> MDQEGQPLLSKDFQQVLLATASGNNSSWTERAVLNNESTDAVKHEPALGQNDVFDLDPLSFDKWVPFLRRALDKNQLDPVIDELENSIEDNFQGLELQLLQDSQMNDKLETSIDEIANIQGMVQDTLSSEISKFQIRLSESANELIVKKQMYVNNKKISLKISEATILITKVVRILELSSKCQELITERKFFKVLQNLDSLEKLYLQEFKNYNFQFLIEIYNSIPFLQKVTKDECINLIRNSLNLNLGKNLIKVGQEFVAIYENELLPQWLETRSKMKLTNFKFNSPIEISMRDESFLAKLNLGEFFQLDDFHDSIMIFQNLNELSVLSGEFNKEYELRKTKLMYPLIWKKNKTAAYQMDSLLRGTGTTPGSTAHDVSTDDPFTQSLSLHFLQDYFLKILGFLLYDINLNKATEFILVDNNYNSTNEFWDGLMDRLSPYLSYFIDEKLKTEEDMIKLKDFLCIYVAILENFKL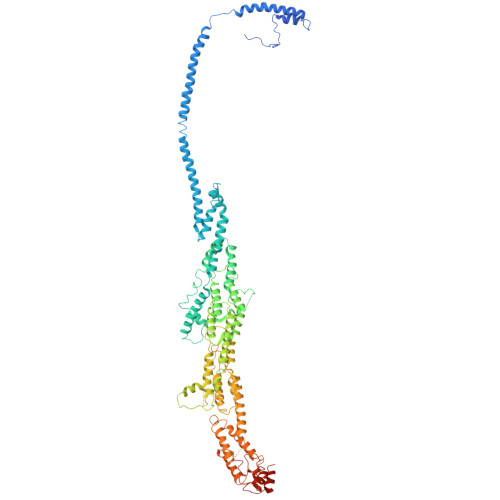NIEPLYKILVSIFEKFCSVSLRAFDDEFQILLNDDDFMPLSINDKTLYEKVLKICWMKEGEHLSLPDPTNGEPFAVTLPFSPLYPMTCTLAKKTYSKITAFLSIFYRHELHTLNNILVKTMDDIFNDIVNKKIRSKLESTSREEIAQILVNLDYFIIAAKEFSNFMTRENILQNPDMEIRLSSIKYLAESRKLAETKLIELIDSKISDILETIEIDWQITEVRQDPDISIIDLAQFLEMMFASTLQNLPYSVQTLLIFREFDSLTRQFMGLLLHDTPSTITHESIMNFEVDVNYLESIIPRIFPSTPGTIDSNGYQSPMTPSTPTFPNANGVDAPTLFENNIKSLEATFMELKQCIELLKTQGKDYNEPEIRLRKYSRIRQEDAALLLSKIQHFVSSVEGANGDDTSVMDSSSIFNSESASVIDSNTSRIAKFFNRR>MSAKAISEQTGKELLYKFICTTSAIQNRFKYARVTPDTDWARLLQDHPWLLSQNLVVKPDQLIKRRGKLGLVGVNLTLDGVKSWLKPRLGQEATVGKATGFLKNFLIEPFVPHSQAEEFYVCIYATREGDYVLFHHEGGVDVGDVDAKAQKLLVGVDEKLNPEDIKKHLLVHAPEDKKEILASFISGLFNFYEDLYFTYLEINPLVVTKDGVYVLDLAAKVDATADYICKVKWGDIEFPPPFGREAYPEEAYIADLDAKSGASLKLTLLNPKGRIWTMVAGGGASVVYSDTICDLGGVNELANYGEYSGAPSEQQTYDYAKTILSLMTREKHPDGKILIIGGSIANFTNVAATFKGIVRAIRDYQGPLKEHEVTIFVRRGGPNYQEGLRVMGEVGKTTGIPIHVFGTETHMTAIVGMALGHRPIPNQPPTAAHTANFLLNASGSTSTPAPSRTASFSESRADEVAPAKKAKPAMPQDSVPSPRSLQGKSTTLFSRHTKAIVWGMQTRAVQGMLDFDYVCSRDEPSVAAMVYPFTGDHKQKFYWGHKEILIPVFKNMADAMRKHPEVDVLINFASLRSAYDSTMETMNYAQIRTIAIIAQGIPEALTRKLIKKADQKGVTIIGPATVGGIKPGCFKIGNTGGMLDNILASKLYRPGSVAYVSRSGGMSNELN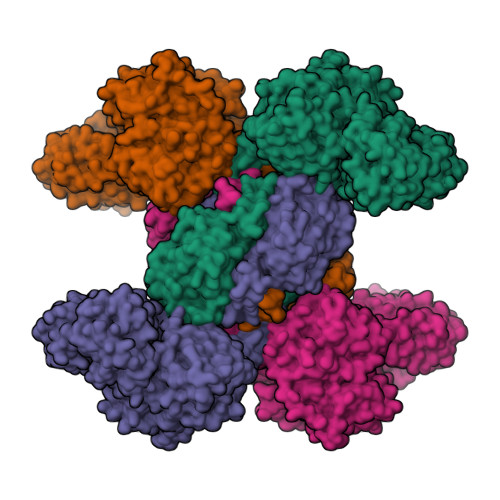NIISRTTDGVYEGVAIGGDRYPGSTFMDHVLRYQDTPGVKMIVVLGEIGGTEEYKICRGIKEGRLTKPIVCWCIGTCATMFSSEVQFGHAGACANQASETAVAKNQALKEAGVFVPRSFDELGEIIQSVYEDLVANGVIVPAQEVPPPTVPMDYSWARELGLIRKPASFMTSICDERGQELIYAGMPITEVFKEEMGIGGVLGLLWFQKRLPKYSCQFIEMCLMVTADHGPAVSGAHNTIICARAGKDLVSSLTSGLLTIGDRFGGALDAAAKMFSKAFDSGIIPMEFVNKMKKEGKLIMGIGHRVKSINNPDMRVQILKDYVRQHFPATPLLDYALEVEKITTSKKPNLILNVDGLIGVAFVDMLRNCGSFTREEADEYIDIGALNGIFVLGRSMGFIGHYLDQKRLKQGLYRHPWDDISYVLPEHMSM[4x]>SNAMHDLNDL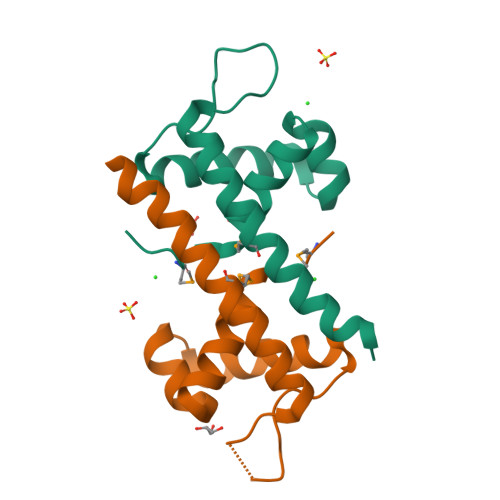YYYAEVVEHGGFSAAARVLGLPKSKLSRRLALLEERLGVRLIQRSTRRFAVTDVGRTYYEHCKAMIEEARAAQESIDLTR[4x]> MYVYPPRIINGTLYKSTDLAEYTRGKILQTLSIVRGELVAD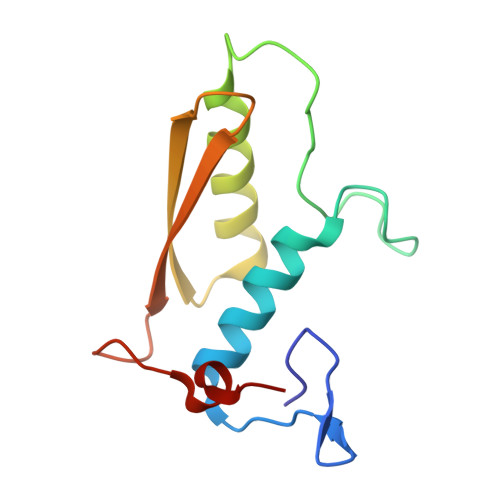PFFGVPLRLFSNINDYQSDVSKIQIILEEEITEAQFIVTGDLKNNGIVSLTVYWAYLGTENIENFEIDTSNIF> SGISLDNSYKMDYPEMGLCIIINNKNFHKSTGMTSRSGTDVDAANLRETFRNLKYEVRNKNDLTREEIVELMRDVSKEDHSKRSSFVCVLL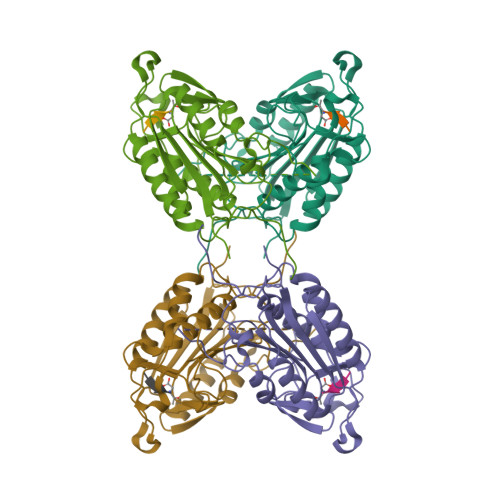SHGEEGIIFGTNGPVDLKKITNFFRGDRCRSLTGKPKLFIIQACRGTALDCGIETDSGVDDDMACHKIPVEADFLYAYSTAPGYYSWRNSKDGSWFIQSLCAMLKQYADKLEFMHILTRVNRKVATEFESFSFDATFHAKKQIPCIVSMLTKELYFYHH N-[(1S)-1-cyclopropylethyl]-N,4-dimethyl-1,3-thiazole-5-carboxamide | C11 H16 N2 O S | 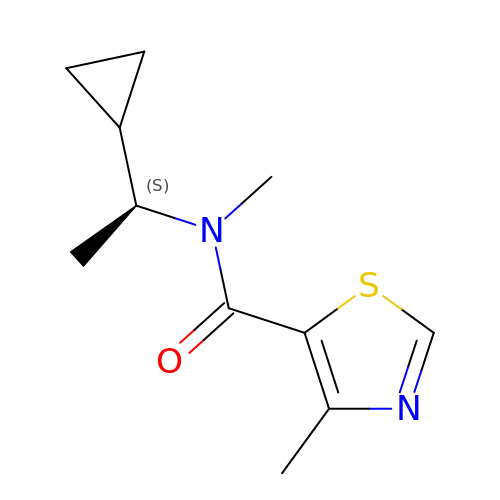BVKVTOXEFCBBBM-QMMMGPOBSA-N> SNAEKKEVPGVDFSITQFVRNLGLEHLMDIFEREQITLRVLVEMGHKELKEIGINAYGHREKLIK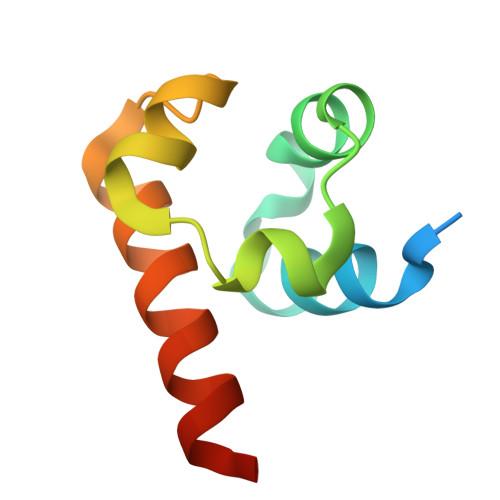GVERLISGQQGL> HHHHHHIEGHIGGAYVLDDSDGLGREFDGIGAVSGGGATSRLLVNYPEPYRSEILDYLFKPNFGASLHILKVEIGGDGQTTDGTEPSHMHYELDENYFRGYEWWLMKEAKKRNPDIILMGLPWSFPGWLGKGFSWPYVNLQLTAYYVVRWILGAKHYHDLDIDYIGIWNERPFDANYIKELRKMLDYQGLQRVRIIASDNLWEPISSSLLLDQELWKVVDVIGAHYPGTYTVWNAKMSGKKLWSSEDFSTINSNVGAGCWSRILNQNYINGNMTSTIAWNLVASYYEELPYGRSGLMTAQE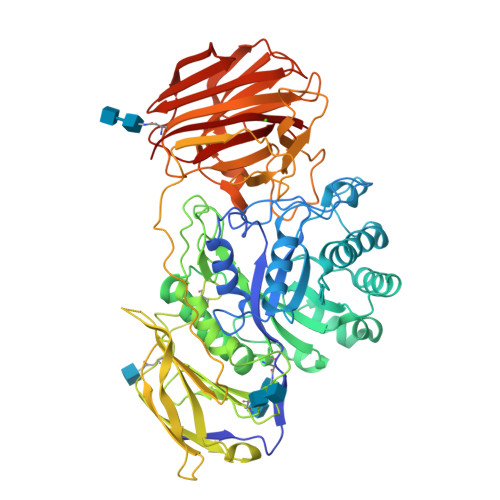PWSGHYVVASPIWVSAHTTQFTQPGWYYLKTVGHLEKGGSYVALTDGLGNLTIIIETMSHQHSMCIRPYLPYYNVSHQLATFTLKGSLREIQELQVWYTKLGTPQQRLHFKQLDTLWLLDGSGSFTLELEEDEIFTLTTLTTGRKGSYPPPPSSKPFPTNYKDDFNVEYPLFSEAPNFADQTGVFEYYMNNEDREHRFTLRQVLNQRPITWAADASSTISVIGDHHWTNMTVQCDVYIETPRSGGVFIAGRVNKGGILIRSATGVFFWIFANGSYRVTADLGGWITYASGHADVTAKRWYTLTLGIKGYFAFGMLNGTILWKNVRVKYPGHGWAAIGTHTFEFAQFDNFRVEAAR>MQGVNIYNISAGTSVDLAAPVTTGDIVTFFSSALNLNAGAGNPNNTTLNLFAENGAYLLHIAFRLQENVIIFNSRQPDGPWLVEQRVSDVANQFAGIDGKAMVTVFDHGDKYQVVI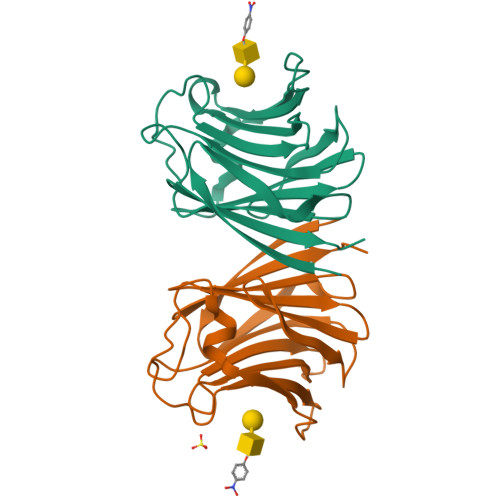NEKTVIQYTKQISGLTSSLSYNATEETSIFSTVVEAVTYTGLA[2x]> MNMYKWVPESIRDSGEGQPSYSNNGDYAPSGPWVAAGIHTMPQSLRDSMRNSIMVTAQARRDVIGPEWGPDGRFTGYASVIGTPDPKPADIVNKFTVERRPVSNGNFQQRVKAGDIVVAPYTSDGKITVKLVAGQKDISSTPDYDYRIDSSLASSAGFVVAGERWY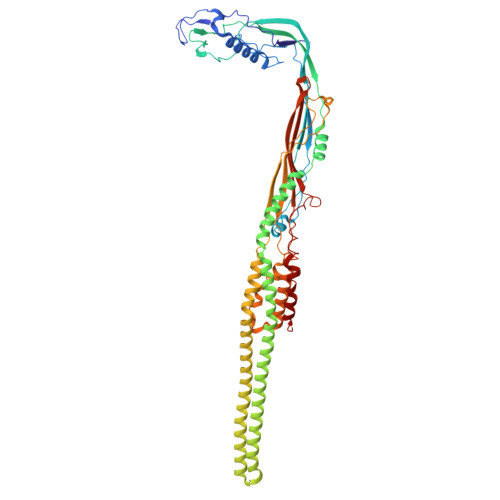YTKRHFIIPRYFQNWRMRRRKYVTGWVMPTFYSPKEIFNRLKDSLVPDTGLVTQVWADNNTKRMDFLTAMAEIPQTLSSFLDALGYLGSLIKDFKRRRFFLNKAHQRIRNKLGVSFAERRSQIVSKYDRKIASARKPAIIVKLRQRKEKALKALDKMRVREEKKMIREFATQAASLWLSFRYEIMPLYYQSQDVLDVIANSTSEFMTSRDFVAKAINIGIPLEWNLDQENLVSQPRHNVMVKSKLSPENNIGKTLSVNPFTTAWELLTLSFVVDWFVNFGDVIAGFTGGYSDDSGATASWRFDDKKVFHLKNIPSAMVIVDINFYTRQVIDPRLCGGLAFSPKLNLFRYLDAMSLSWNRSRLKISRAT> GPDSMLKSKTFLKKTRAGGVMKIVREHYLRDDIGCGAPGCAACGGAHEGPALEPQPQDPASSVCPQPHYLLPDTNVLLHQIDVLEDPAIRNVIVLQTVLQEVRNRSAPVYKRIRDVTNNQEKHFYTFTNEHHRETYVEQEQGENANDRNNRAIRVAAKWYNEHLKKMSADNQLQVIFITNDRRNKEKAIEEGIPAFTCEEYVKSLTANPELIDRL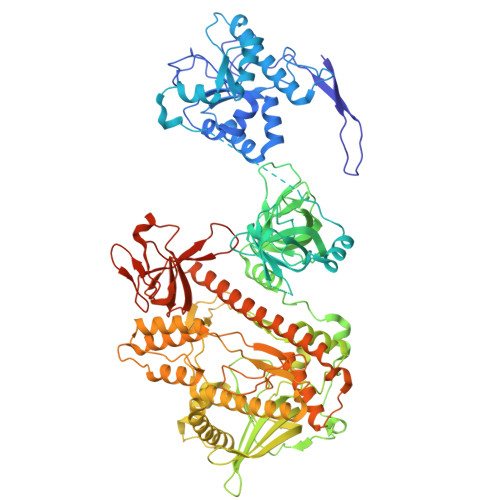ACLSEEGNEIESGKIIFSEHLPLSKLQQGIKSGTYLQGTFRASRENYLEATVWIHGDNEENKEIILQGLKHLNRAVHEDIVAVELLPKSQWVAPSSVVLHDEGQNEEDVEKEEETERMLKTAVSEKMLKPTGRVVGIIKRNWRPYCGMLSKSDIKESRRHLFTPADKRIPRIRIETRQASTLEGRRIIVAIDGWPRNSRYPNGHFVRNLGDVGEKETETEVLLLEHDVPHQPFSQAVLSFLPKMPWSITEKDMKNREDLRHLCICSVDPPGCTDINDALHCRELENGNLEVGVHIADVSHFIRPGNALDQESARRGTTVYLCEKRIDMVPELLSSNLCSLKCDVDRLAFSCIWEMNHNAEILKTKFTKSVINSKASLTYAEAQLRIDSANMNDDITTSLRGLNKLAKILKKRRIEKGALTLSSPEVRFHMDSETHDPIDLQTKELRETNSMVEEFMLLANISVAKKIHEEFSEHALLRKHPAPPPSNYEILVKAARSRNLEIKTDTAKSLAESLDQAESPTFPYLNTLLRILATRCMMQAVYFCSGMDNDFHHYGLASPIYTHFTSPIRRYADVIVHRLLAVAIGADCTYPELTDKHKLADICKNLNFRHKMAQYAQRASVAFHTQLFFKSKGIVSEEAYILFVRKNAIVVLIPKYGLEGTVFFEEKDKPNPQLIYDDEIPSLKIEDTVFHVFDKVKVKIMLDSSNLQHQKIRMSLVEPQIPGISIPTDTSNMDLNGPKKKKMKLGK> 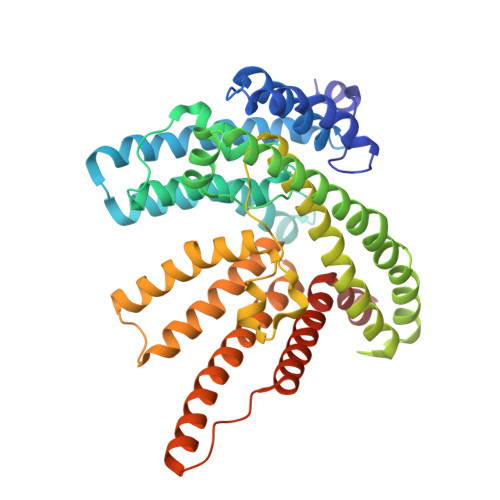MIDFLKQLPHLEPYGNPFYFIYLGIALLPIFIGLFFKKRFAIYECLVSITFIVLALTGTHASQILALLFYIVWQIIWVYSYKRYRSQRDNKWVFYLHSFLVVLPLILVKVEPTINGTQSLLNFLGISYLTFRAVGMIIEMRDGVLKEFTLGEFLRFMLFMPTFTSGPIDRFKRFNEDYQSIPNRDELLNMLEQAVKYIMLGFLYKFVLAQIFGSMLLPPLKAQALSQGGIFNLPTLGVMYVYGFDLFFDFAGYSMFALAVSNLMGIKSPINFDKPFISRDMKEFWNRWHMSLSFWFRDFVFMRLVIVLMRNKVFKNRNTTSNVAYIINMMVMGFWHGITWYYIAYGIFHGIGLVINDAWLRKKKTINKDRKKAGLKPLPENKWTKALGIFITFNTVMLSFLIFSGFLNDLWFTKKLEHHHHHHHH> MALKAQNTISGKEGRLFLDGEEMAHIKTFEANVEKNKSEVNIMGRRMTGHKTTGANGTGTATFYKVTSKFVLLMMDY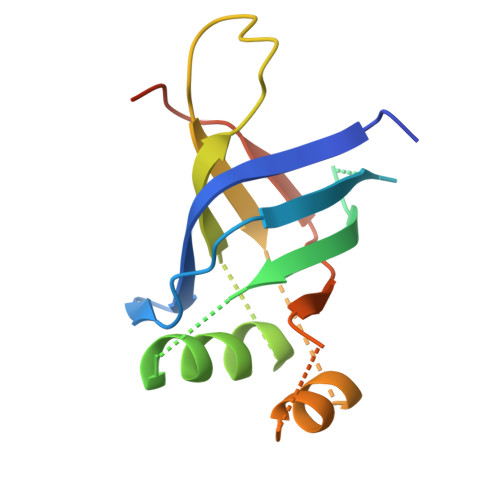VKKGSDPYFTLQAVLDDQSSGRGTERVTLYDVNFDSAKIASLDVDSEALEEEVPFTFEDFDVPEKLSDTFLEHHHHHH>[2x]MTDGLNQLYNLVAQDYALTDTIEALSRMLHRGTIPLDTFVKQGRELARQQFLVRWHIQRITSPLS;>[2x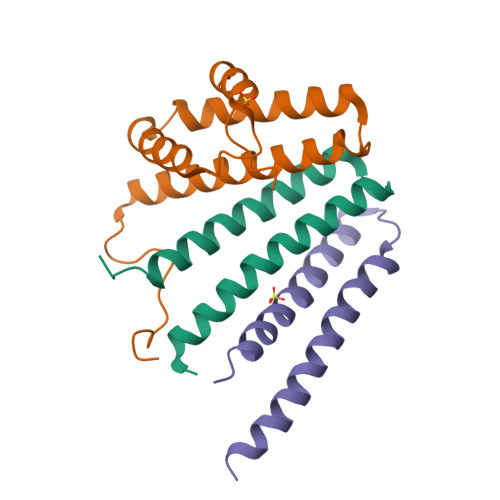]GAMDISQLFHDEVPLFDNSITSKDKEVIETLSEIYSIVITLDHVEKAYLKDSIDDTQYTNTVDKLLKQFKVYLNSQNKEEINKHFQSIEAFADTYNITASNAITRLERGIPITAEH;>[2x]ASWQDYHSEFSKKYGDIALKKKLEQNTKKLDEESSQLETTTRSIDSADDLDQFIKNYLDIRTQYHLRREKLATWDKQGNLKY>[2x]AMRQCAIYGKGGIGKSTTTQNLVAALAEMGKKVMIVGCNPKADSTRLILHSKAQNTIMEMAAEAGTVEDLELEDVLKAGYGGVKCVESGGPEPG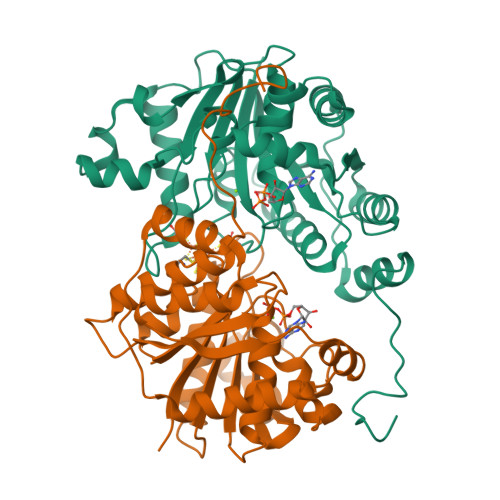VGCAGRGVITAINFLEEEGAYEDDLDFVFYDVLGDVVCGGFAMPIRENKAQEIYIVCSGEMMAMYAANNISKGIVKYANSGSVRLGGLICNSRNTDREDELIIALANKLGTQMIHFVPRDNVVQRAEIRRMTVIEYDPKAKQADEYRALARKVVDNKLLVIPNPITMDELEELLMEFGIMEVEDESIVGKTAEEV> MQEYTNHSDTTFALRNISFRVPGRTLLHPLSLTFPAGKVTGLIGHNGSGKSTLLKMLGRHQPPSEGEILLDAQPLESWSSKAFARKVAYLPQQLPPAEGMTVRELVAIGRYPWH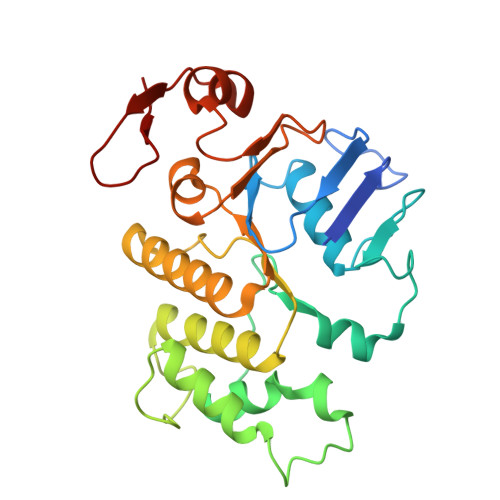GALGRFGAADREKVEEAISLVGLKPLAHRLVDSLSGGERQRAWIAMLVAQDSRCLLLDEPTSALDIAHQVDVLSLVHRLSQERGLTVIAVLHDINMAARYCDYLVALRGGEMIAQGTPAEIMRGETLEMIYGIPMGILPHPAGAAPVSFVY>[3x]M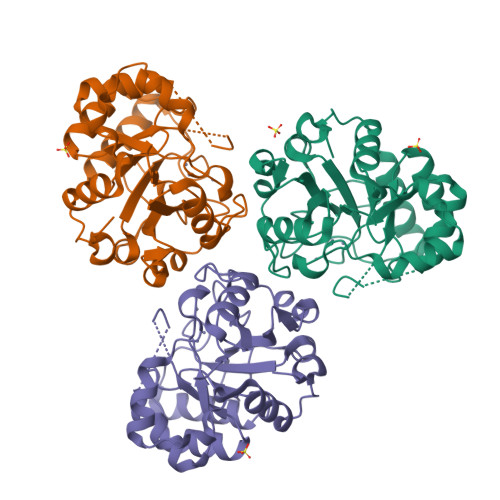YPVDLHMHTVASTHAYSTLSDYIAQAKQKGIKLFAITDHGPDMEDAPHHWHFINMRIWPRVVDGVGILRGIEANIKNVDGEIDCSGKMFDSLDLIIAGFHEPVFAPHDKATNTQAMIATIASGNVHIISHPGNPKYEIDVKAVAEAAAKHQVALEINNSSFLHSRKGSEDNCREVAAAVRDAGGWVALGSDSHTAFTMGEFEECLKILDAVDFPPERILNVSPRRLLNFLESRGMAPIAEFADL>[2x]MGENMKKKVVIIGGGAAGMSAASRVKRLKPEWDVKVFEATEWVSHAPCGIPYVVEGLSTPDKLMAAGPEVFIKKRGIDLHLNAEVIEVDTGYVRVRENGGEKSYEWDYLVFANGASPQVPAIE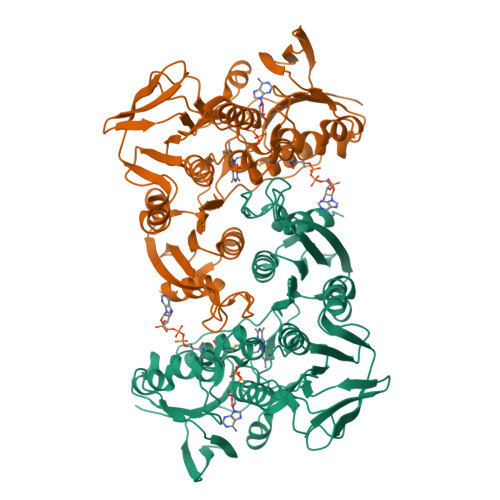GVNLKGVFTADLPPDALAIREYMEKYKVENVVIIGGGYIGIEMAEAFAAQGKNVTMIVRGERVLRRSFDKEVTDILEEKLKKHVNLRLQEITMKIEGEERVEKVVTDAGEYKAELVILATGIKPNIELAKQLGVRIGETGAIWTNEKMQTSVENVYAAGDVAETRHVITGRRVWVPLAPAGNKMGYVAGSNIAGKELHFPGVLGTAVTKFMDVEIGKTGLTEMEALKEGYDVRTAFIKASTRPAYYPGGREIWLKGVVDNETNRLLGVQVVGSDILPRIDTAAAMLMAGFTTKDAFFTDLAYAPPFAPVWDPLIVLARVLKFLEHHHHHH>[4x]SWMANQFFLLEEYTGSDYQYVGKLHSDQDRGDGSLKYILSGDGAGDLFIINENTGDIQATKRLDREEKPVYILRAQAVNRRTGR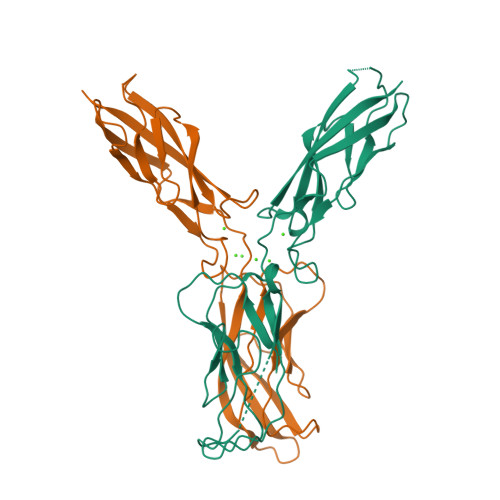PVEPESEFIIKIHDINDNEPIFTKDVYTATVPEMADVGTFVVQVTATDADDPTYGNSAKVVYSILQGQPYFSVESETGIIKTALLNMDRENREQYQVVIQAKDMGGQMGGLSGTTTVNITLTD[9-[2-carboxy-5-[2-[2-(5-oxidanylpentoxy)ethoxy]ethylcarbamoyl]phenyl]-6-(dimethylamino)xanthen-3-ylidene]-dimethyl-azanium | C34 H42 N3 O7 | 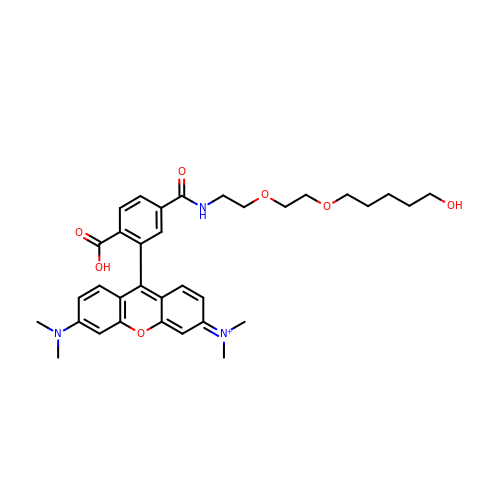JWWZUBNFGVWRTE-UHFFFAOYSA-O>[4x]MPIEPQSDAHVLKSRLEWGEPAFTILDVRDRSTYND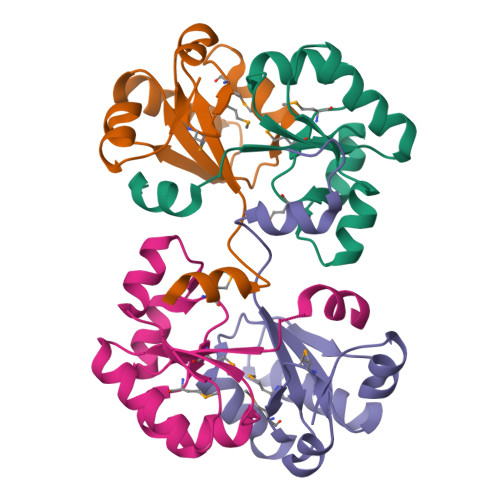GHIMGAMAMPIEDLVDRASSSLEKSRDIYVYGAGDEQTSQAVNLLRSAGFEHVSELKGGLAAWKAIGGPTELEHHHHHH> GSEDLIDGIIFAANYLGSTQLLSERNPSKNIRMMQAQEAVSRVKRMQKAAKIKKKANSEGDAQTLTEVDLFISTQRIKVLNADTQETMMDHALRTISYIADI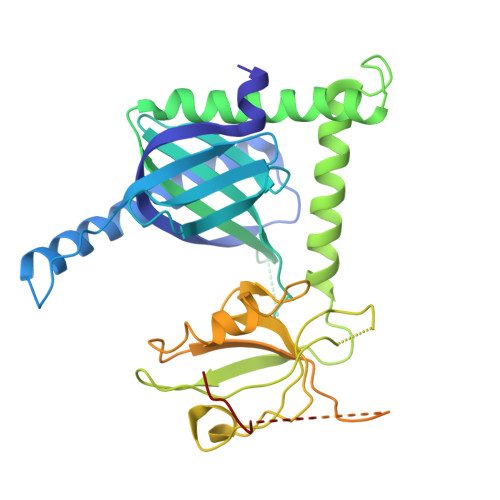GNIVVLMARRRMPRSASQDCIETTPGAQEGKKQYKMICHVFESEDAQLIAQSIGQAFSVAYQEFLRANGINPEDLSQKEYSDIINTQEMYNDDLIHFSNSENCKELQLEKHKGEILGVVVVESGWGSILPTVILANMMNGGPAARSGKLSIGDQIMSINGTSLVGLPLATCQGIIKGLKNQTQVKLNIVSCPPVTTVLIKRPDLKYQLGFSVQNGIICSLMRGGIAERGGVRVGHRIIEINGQSVVATAHEKIVQALSNSVGEIHMKTMPAAMFRLLTGQETPLYI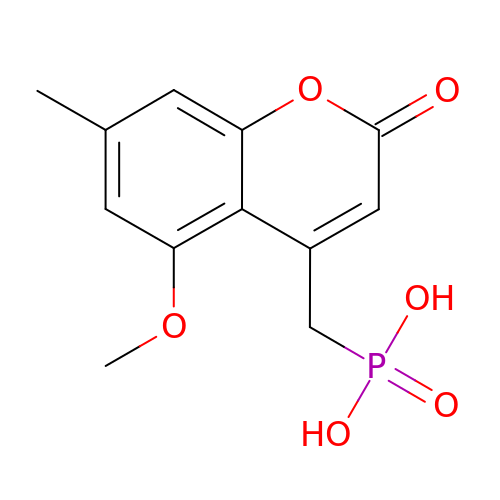[(5-methoxy-7-methyl-2-oxo-2H-1-benzopyran-4-yl)methyl]phosphonic acid | C12 H13 O6 P | OPIKUXFTGMKVTE-UHFFFAOYSA-N> IEEVMKTVANTVESEIRAELGVIPSLNAAETGATSNTTPEEAIQTRAVINQHGTSETLVENFLGRAALVMMKDFEYKNHVTGTQKVQQNFFKWTINTRSYVQLRRKFELFTYIRFDSEITIVPTIRLYTSTGASYSGLPNLTLQAMFVPVGAPTPKSQDSYEWQSACNPSVFFKIDDPPARMTIPFMCINSAYGMFYDGFAGFEKTANGLYGINPANTMGNLCIRVVNAYQPVQYTITIRIYLKPKHIKAWVPRPPRTMPYMSIANTNYTGHSSAPNNVNAIVGNRTNITTMPNDIVT;> SDRVLQLKLGNSAIVTQEAANMCCAYGEWPSYLPDNEATAIDKPTQPETSTDRFYTLKSVKWEGTSTGWWWKLPDALNQTGMFGQNVQYHYLYRSGFLCHVQCNATKFHQGALLVVAIPEHQLGKYNTGTSASFDDVMKGKTGGVFTHPYVLDDGTSLACSLIFPHQWINLRTNNSATIMLPWMNCAPMDFALRHNQWTLAIIPVVPLNTSGGTTMVPITVSIAPMCCEFNGLRNAIT;> GVPTYLLPGSSQFMTTDDHSSAPAFPDFSPTPEIHIPGRVHNMLELVQVESMMEI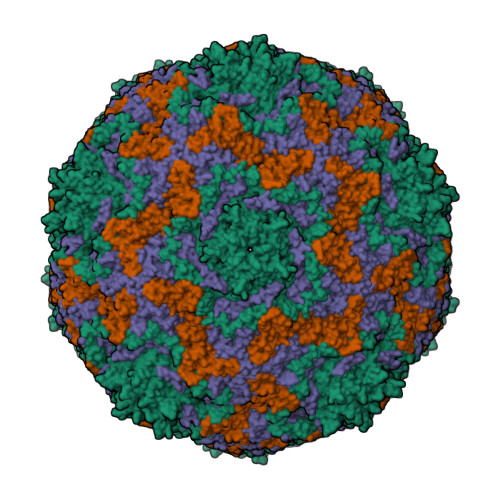NNVAGSSGMERLRVEISVQTDMDALLFNIPLDIQLDGPLRSTLLANIARYYTHWSGSMEMTFMFCGSFMATGKVILCYTPPGGSCPTDRESAMLGTHIVWDFGLQSSITLVIPWISGSHFRMFNSDAKSINANVGYVTCFMQTNLIVPKEAATSTYIIGFAAAKNDFSLRLMRDSPDIGQSQQLEGATAAFQ;> INFYKDSYAASASKQDFSQDPSKFTEPVADALKAGAPVL> DYPKTGVATSIVEKIERAEFNTAGRKPTVLLRIADFIAAMNGMDAKQDMQALWDAEIAIMNGRAQTTIISYITKYRNAIREAFGDDHPMLKIATGDAAMYDEARRVKMEKIANKHGALITFENYRQVLKICEDCLKSSDPLMIGIGLIGMTGRAPYEVFTQAEFSPAPYGKGVSKWSILFNGQAKTKQGEGTKFGITYEIPVLTRSETVLAAYKRLRESGQGKLWHGMSIDDFSSETRLLLRDTVFNLFEDVWPK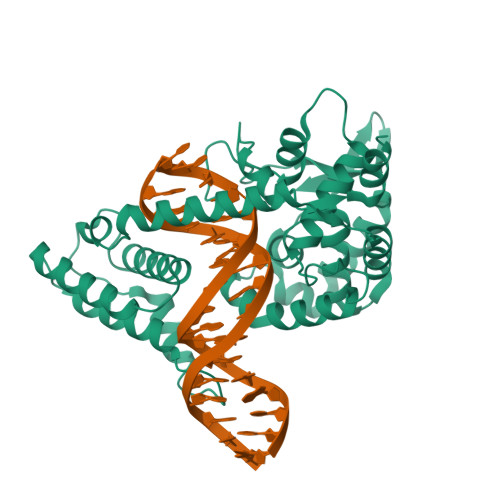EELPKPYGLRHLYAEVAYHNFAPPHVTKNSYFAAILGHNNNDLETSLSYMTYTLPEDRDNALARL>MMKNILAIQSHVVYGHAGNSAAEFPMRRLGANVWPLNTVQFSNHTQYGKWTGCVMPPSHLTEIVQGIAAIDKLHTCDAVLSGYLGSAEQGEHILGIVRQVKAANPQAKYFCDPVMGHPEKGCIVAPGVAEFHVRHGLPASDIIAPNLVELEILCEHAVNNVEEAVLAARELIAQGPQIVLVKHLARAGYSRDRFEMLLVTADEAWHISRPLVDFGMRQPVGVGDVTSGLLLVKLLQGATLQEALEHVTAAVYEIMVTTKAMQEYELQ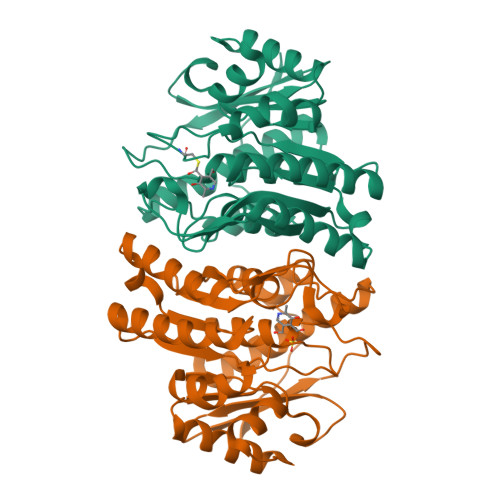VVAAQDRIAKPEHYFSATKL[2x]> MPFTIDSARGIFPNTLAADVVPATIARFSQLNAEDQLALIWFAYLEMGKTLTIAAPGAASMQLAENALKEIQAMGPLQQTQAMCDLANRADTPLCRTYASW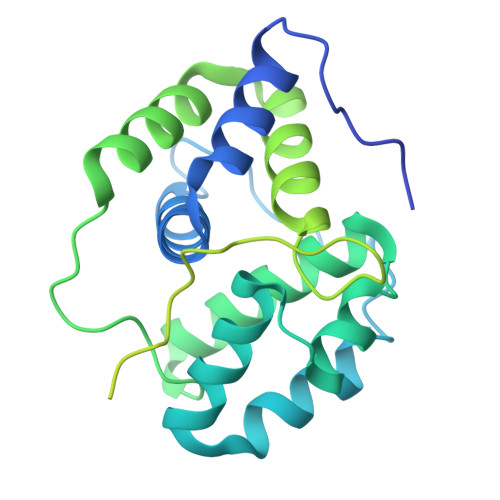SPNIKLGFWYRLGELMEQGFVAPIPAGYQLSANANAVLATIQGLESGQQITVLRNAVVDMGFTAGKDGKRIAEPVVPPQDTASRTKVSIEGVTNATVLNYMDNLNANDFDTLIELFTSDGALQPPFQRPIVGKENVLRFFREECQNLKLIPERGVTEPAEDGFTQIKVTGKVQTPWFGGNVGMNIAWRFLLNPEGKIFFVAIDLLASPKELLNFAR>GDQLTHVVEEVKTYDLVWRSIKNLWEDVQRTFETPWCRVDVLLLQSDLANFLRRADELPRAVKQFEMYKSLFSQVNMLTSVNKILVELKDGALKPRHWNMIFRDIGKRQIQKNLLDKLEFSLKDVMVLNLTLNEILLTKIIERAQKEFVIEKSLNRIKKFWKEAQYEVIEHSSGLKLVREWDVLEQACKEDLEELVSMKASNYYKIFEQDCLDLESKLTKLSEIQVNWVEVQFYWLDLYGILGENLDIQNFLPLETSKFKSLTSEYKMITTRAFQLDTTIEVIHIPNFDTTLKLTIDSLKMIKSSLSTFLERQRRQFPRFYFLGNDDLLKIIGSGKHHDQVSKFMKKMFGSIESIIFFEDSITGVRSVEGEVLNLNEKIELKDSIQAQEWLNILDTEIKLSVFTQFRDCLGQLKDGTDIEVVVSKYIFQAILLSAQVMWTELVEKCLQTNEFSKYWKEVDMKIKGLLDKLNKSSDNVKKKIEALLVEYLHFNNVIGQLKNCSTKEEARLLWAKVQKFYQKNDTLDDLNSVFISQSGYLLQYKFEYIGIPERLIYTPLLLVGFATLTDSLHQKYGGCFFGPAGTGKTETVKAFGQNLGRVVVVFNCDDSFDYQVLSRLLVGITQIGAWGCFDEFNRLDEKVLSAVSANIQQIQNGLQVGKSHITLLEEETPLSPHTAVFITLNPGYNGRSELPENLKKSFREFSMKSPQSGTIAEMILQIMGFEDSKSLASKIVHFLELLSSKCSSMNHYHFGLRTLKGVLRNCSPLVSEFGEGEKTVVESLKRVILPSLGDTDELVFKDELSKIFDSAGTPLNSKAIVQCLKDAGQRSGFSMSEEFLKKCMQFYYMQKTQQALILVGKAGCGKTATWKTVIDAMAIFDGHANVVYVIDTKVLTKESLYGSMLKATLEWRDGLFTSILRRVNDDITGTFKNSRIWVVFDSDLDPEYVEAMNSVLDDNKILTLPNGERLPIPPNFRILFETDNLDHTTPATITRCGLLWFSTDVCSISSKIDHLLNKSYEALDNKLSMFELDKLKDLISDSFDMASLTNIFTCSNDLVHILGVRTFNKLETAVQLAVHLISSYRQWFQNLDDKSLKDVITLLIKRSLLYALAGDSTGESQRAFIQTINTYFGHDSQELSDYSTIVIANDKLSFSSFCSEIPSVSLEAHEVMRPDIVIPTIDTIKHEKIFYDLLNSKRGIILCGPPGSGKTMIMNNALRNSSLYDVVGINFSKDTTTEHILSALHRHTNYVTTSKGLTLLPKSDIKNLVLFCDQINLPKLDKYGSQNVVLFLRQLMEKQGFWKTPENKWVTIERIHIVGACNPPTDPGRIPMSERFTRHAAILYLGYPSGKSLSQIYEIYYKAIFKLVPEFRSYTEPFARASVHLYNECKARYSTGLQSHYLFSPRELTRLVRGVYTAINTGPRQTLRSLIRLWAYEAWRIFADRLVGVKEKNSFEQLLYETVDKYLPNQDLGNISSTSLLFSGLLSLDFKEVNKTDLVNFIEERFKTFCDEELEVPMVIHESMVDHILRIDRALKQVQGHMMLIGASRTGKTILTRFVAWLNGLKIVQPKIHRHSNLSDFDMILKKAISDCSLKESRTCLIIDESNILETAFLERMNTLLANADIPDLFQGEEYDKLLNNLRNKTRSLGLLLDTEQELYDWFVGEIAKNLHVVFTICDPTNNKSSAMISSPALFNRCIINWMGDWDTKTMSQVANNMVDVVPMEFTDFIVPEVNKELVFTEPIQTIRDAVVNILIHFDRNFYQKMKVGVNPRSPGYFIDGLRALVKLVTAKYQDLQENQRFVNVGLEKLNESVLKVNELNKTLSKKSTELTEKEKEARSTLDKMLMEQNESERKQEATEEIKKILKVQEEDIRKRKEVVMKSIQDIEPTILEAQRGVKNIKKQQLTEIRSMVNPPSGVKIVMEAVCAILGYQFSNWRDIQQFIRKDDFIHNIVHYDTTLHMKPQIRKYMEEEFLSDPNFTYETINRASKACGPLYQWVNAQINFSKVLENVDPLRQEMKRIEFESLKTKANLLAAEEMTQDLEASIEVSKQKYSLLIRDVEAIKTEMSNVQANLDRSISLVKSLTFEKERWLNTTKQFSKTSQELIGNCIISSIYETYFGHLNERERGDMLVILKRLLGKFAVKYDVNYRFIDYLVTLDEKMKWLECGLDKNDYFLENMSIVMNSQDAVPFLLDPSSHMITVISNYYGNKTVLLSFLEEGFVKRLENAVRFGSVVIIQDGEFFDPIISRLISREFNHAGNRVTVEIGDHEVDVSGDFKLFIHSCDPSGDIPIFLRSRVRLVHFVTNKESIETRIFDITLTEENAEMQRKREDLIKLNTEYRLKLKNLEKRLLEELNNSQGNMLENDELMVTLNNLKKEAMNIEKKLSESEEFFPQFDNLVEEYSIIGKHSVKIFSMLEKFGQFHWFYGISIGQFLSCFKRVFIKKSRETRAARTRVDEILWLLYQEVYCQFSTALDKKFKMIMAMTMFCLYKFDIESEQYKEAVLTMIGVLSESSDGVPKLTVDTNDDLRYLWDYVTTKSYISALNWFKNEFFVDEWNIADVVANSENNYFTMASERDVDGTFKLIELAKASKESLKIIPLGSIENLNYAQEEISKSKIEGGWILLQNIQMSLSWVKTYLHKHVEETKAAEEHEKFKMFMTCHLTGDKLPAPLLQRTDRVVYEDIPGILDTVKDLWGSQFFTGKISGVWSVYCTFLLSWFHALITARTRLVPHGFSKKYYFNDCDFQFASVYLENVLATNSTNNIPWAQVRDHIATIVYGGKIDEEKDLEVVAKLCAHVFCGSDNLQIVPGVRIPQPLLQQSEEEERARLTAILSNTIEPADSLSSWLQLPRESILDYERLQAKEVASSTEQLLQEM[2x];>GMTNWQQQLPLTDTQKNELDKSVLRYLNWNYKQTVRHEHAQDYESVRHAIVTLSGFLLQESVDRQEFISNNDTSNESMVDIDELLLPKKWNSIVRLQKKIIELEQNTETLVSQIKDLNTQVSELAQFKPTTSNGTSAHNVLKWIPRNLPSCLINVESSVTSVKLHPNLPIVFVATDHGKLYAFDLFNYTIPLASLQSHTKAITSMDVLFTNYTNSSKKNYLVIVTASKDLQIHVFKWVSEECKFQQIRSLLGHEHIVSAVKIWQKNNDVHIASCSRDQTVKIWDFHNGWSLKTFQPHSQWVRSIDVLGDYIISGSHDTTLRLTHWPSGNGLSVGTGHEFPIEKVKFIHFIEDSPEIRFRTPSTDRYKNWGMQYCVSASRDRTIKIWEIPLPTLMAHRAPIPNPTDSNFRCVLTLKGHLSWVRDISIRGQYLFSCADDKSVRCWDLNTGQCLHVWEKLHTGFVNCLDLDVDFDSNVTPRQMMVTGGLDCKSNVFMR[4x]

Cytoplasmic dynein-1 (dynein) is the main minus-end-directed microtubule motor responsible for transporting vesicles, protein complexes, RNAs, organelles, and viruses along microtubules. Dynein is autoinhibited and undergoes conformational changes to form an active complex that consists of one or two dynein dimers, the dynactin complex, and activating adapter(s). Dynein function in vivo also requires Lis1, which is an essential positive regulator of dynein, as shown by genetic studies in many organisms. Lis1 is required for active dynein complexes to form, but how it enables this is unclear.

Using this subset of particles, we solved a structure of two dynein motor domains in complex with two Lis1 dimers to 4.1 Å. We called this structure ‘Chi’ because the dynein conformation resembles the Greek letter Chi, and because Chi follows Phi in the Greek alphabet. In our structure, two dynein motor domains, each bound by a Lis1 dimer, come together through dynein–Lis1 interactions which, to the best of our knowledge, have not been previously reported. This arrangement is consistent with previous studies that have reported the binding of two Lis1 dimers to dynein in solution. In Chi, the Lis1 proteins bound to the dynein motor domains act as wedges that keep the two dyneins apart, preventing most of the interactions that stabilize Phi. The one exception is a contact between dynein’s stalk helices, which acts as a hinge where Phi opens to accommodate Lis1 and transition to Chi. The dynein–dynein Phi contacts that are disrupted in Chi are replaced by new contacts between Lis1 bound to sitering on one dynein and the AAA5 and AAA6 domains of the opposite dynein. The AAA5 and AAA6 Chi-specific interactions involve residues on Lis1’s β-propeller that are different from those involved in all previously characterized Lis1–dynein and Lis1–Lis1 contacts. The Lis1 bound to sitestalk does not interact with the opposite dynein molecule in Chi. In contrast, in Chi, the linker is disengaged from AAA2 and AAA3 and shifted towards the opposing dynein molecule; this accommodates the increased distance between the motor domains caused by the presence of Lis1. The major features of the Chi structure—the disruption of most Phi-stabilizing interactions, a shift in the linker–linker interface, and the dependence of these on the presence of Lis1 and new interactions between Lis1 and dynein—suggest that Chi is an early intermediate in the activation of dynein that provides a mechanistic explanation for the role of Lis1 in this process.> MYVAVKGGEKAIDAAHALQESRRRGDTDLPELSVAQIEQQLNLAVDRVMTEGGIADRELAALALKQASGDNVEAIFLLRAYRTTLAKLAVSEPLDTTGMRLERRISAVYKDIPGGQLLGPTYDYTHRLLDFTLLANGEAPTLTTADSEQQPSPHVFSLLARQGLAKFEEDSGAQPDDITRTPPVYPCSRSSRLQQLMRGDEGYLLALAYSTQRGYGRNHPFAGEIRSGYIDVSIVPEELGFAVNVGELLMTECEMVNGFIDPPGEPPHFTRGYGLVFGMSERKAMAMALVDRALQAPEYGEHATGPAQDEEFVLAHADNVEVAGFVSHLKLP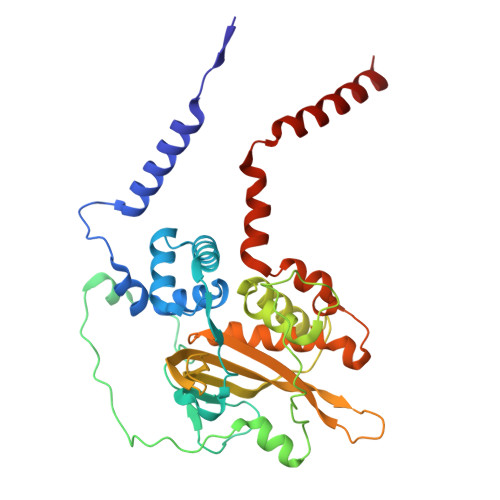HYVDFQAELELLKRLQQEQNHG>[2x]MRDHRKIGKQLDLYHMQEEAPGMVFWHNDGWTIFRELEVFVRSKLKEYQYQEVKGPFMMDRVLWEKTGHWDNYKDAMFTTSSENREYCIKPMNCPGHVQIFNQGLKSYRDLPLRMAEFGSCHRNEPSGSLHGLMRVRGFTQDDAHIFCTEEQIRDEVNGCIRLVYDMYSTFGFEKIVVKLSTRPEKRIGSDEMWDRAEADLAVALEENNIPFEYQLGEGAFFGPKIEFTLYDCLDRAWQCGTVQLDFSLPSRLSASYVGEDNERKVPVMIHRAILGSMERFIGILTEEFAGFFPTWLAPVQVVIMNITDSQSEYVNELTQKLSNAGIRVKADLRNEKIGFKIREHTLRRVPYMLVCGDKEVESGKVAVRTRRGKDLGSMDVNEVIEKLQQEIRSRSLKQLEELEHHHHHH

Aminoacyl-tRNA synthetases (AARSs), a family of essential protein synthesis enzymes, are attractive targets for drug development. Here we present five unusual crystal structures showing that threonyl-tRNA synthetase (ThrRS) is covalently inhibited by a natural product, obafluorin (OB). OB contains a β-lactone ring with a 2,3-dihydroxybenzamidyl moiety attached to the α position and a 4-nitrobenzyl moiety attached to the β position. When ThrRS catalyzes tRNA aminoacylation, the Zn2+ ion recognizes and binds l-threonine, assisting in the l-threonine activation reaction.

To test the mutually exclusive effect between OB and ATP, we engineered a ThrRS_Y462F mutant that mutated Tyr462 to phenylalanine to avoid covalent bonding with OB. As a result, in the TSA experiment, OB only increased the Tm of ThrRS_Y462F by 2.6 °C, while 36j still increased the Tm of ThrRS_Y462F by 29.7 °C. Consistently, OB failed to inhibit the activity of ThrRS_Y462F in the ATP hydrolysis assay up to 5 μM. More interestingly, when we cocrystallized ThrRS_Y462F with OB and ATP, ATP was visible in the active site of ThrRS together with two cobound Mg2+ ions. No densities for OB were observed in the active center. Without the binding of OB, the conformation of Tyr313 of ThrRS_Y462F was in a position that would clash with OB as it was in the ThrRS-OB complexes. In addition, compared with the ThrRS_Y462F-ATP structure, OB induced a significant conformational change to the outer side of the active cleft, which was similar to that induced by another potent ThrRS inhibitor, borrelidin. Therefore, OB prevents ThrRS from binding to all three substrates, including l-threonine, tRNA, and ATP.>[8x]LPNITILATGGTIAGGGDSATKSNYTAGKVGVENLVNAVPQLKDIANVKGEQVVNIGSQDMNDNVWLTLAKKINTDCDKTDGFVITHGTDTMEETAYFLDLTVKCDKPVVMVGAMRPSTSMSADGPFNLYNAVVTAADKASANRGVLVVMNDTVLDGRDVTKTNTTDVATFKSVNYGPLGYIHNGKIDYQRTPARKHTSDTPFDVSKLNELPKV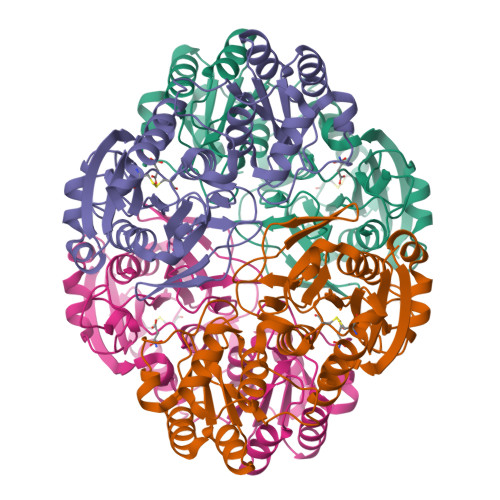GIVYNYANASDLPAKALVDAGYDGIVSAGVGNGNLYKSVFDTLATAAKNGTAVVRSSRVPTGATTQDAEVDDAKYGFVASGTLNPQKARVLLQLALTQTKDPQQIQQIFNQY> GGCUUAUCAAGAGAGGUGGAGGGACU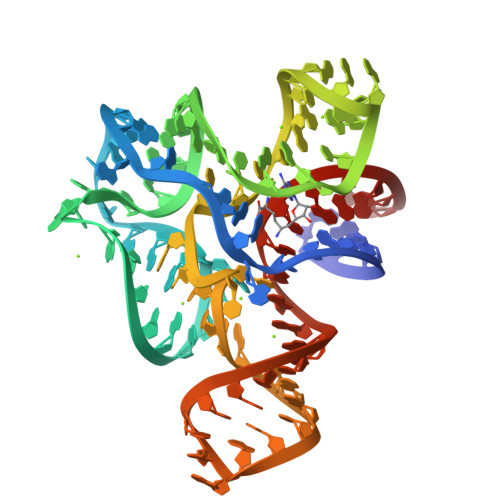GGCCCGACGAAACCCGGCAACCAGAAAUGGUGCCAAUUCCUGCAGCGGAAACGUUGAAAGAUGAGCCG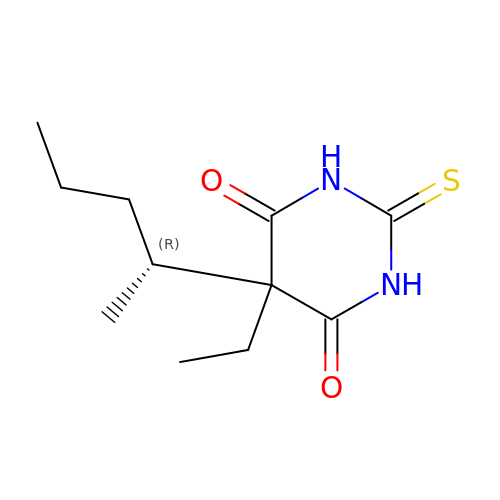5-ethyl-5-[(2R)-pentan-2-yl]-2-thioxodihydropyrimidine-4,6(1H,5H)-dione | C11 H18 N2 O2 S | IUJDSEJGGMCXSG-SSDOTTSWSA-N>MSQSVSERTRIKSDRYESGVIPYAKMGYWDAAYSVKDTDILALFRITPQPGVDPVEAAAAVAGESSTATWTVVWTDLLTACERYRAKAYRVDPVPNSTDVYFAFIAYECDLFEEASLSNLTASIIGNVFGFKAISALRLEDMRIPHSYLKTFQGPATGIIVERERLNKYGTPLLGATVKPKLGLSGKNYGRVVYEGLKGGLDFLKDDENINSQPFMRWRERFLNCLEGINRAAAATGEVKGSYLNITAATMEEVYKRAEYAKAIGSVVVMIDLVMGYTAIQSIAYWARENDMLLHLHRAGNSTYARQKNHGINFRVICKWMRMSGVDHIHAGTVVGKLEGDPLMIKGFYDILRLTELEVNLPFGIFFEMDWASLRRCMPVASGGIHCGQMHQLIHYLGDDVVLQFGGGTIGHPDGIQAGATANRVALEAMVLARNEGADYFNNQVGPQILRDAAKTCGPLQTALDLWKDISFNYTSTDTADFAETATANR[8x];>[8x]MRLTQGCFSFLPDLTDQQIEKQVACAMSRGLAMNVEWTDDPHPRNNYWELWGLPLFDIKDPATVMFELNEARKSCAAGYIRMNAFDASYGTESCVMSFITNRPANEPGFYLDRTEGVGRQIVYS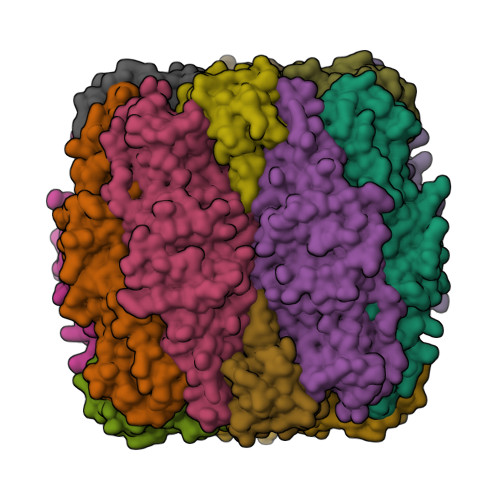IKSYSVQANPEGSRY>[4x]AGDAEAGQGKVAVCGACHGVDGNSPAPNFPKLAGQGERYLLKQLQDIKAGSTPGAPEGVGRKVLEMTGMLDPLSDQDLEDIAAYFSSQKGSVGYADPALAKQG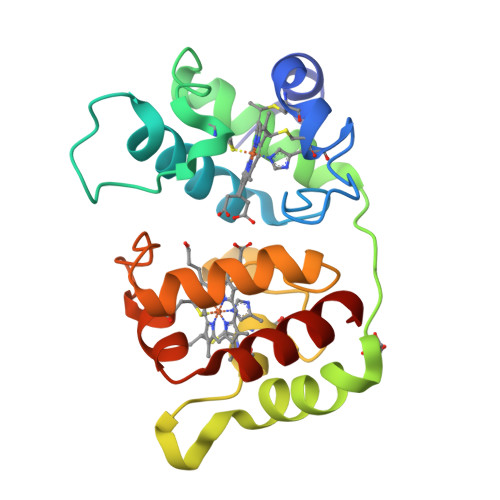EKLFRGGKLDQGMPACTGCHAPNGVGNDLAGFPKLGGQHAAYTAKQLTDFREGNRTNDGDTMIMRGVAAKLSNKDIEALSSYIQGLH>MAAAVTVEEVRRAQRAEGPATVLAIGTATPANCVYQADYPDYYFRITKSEHMVELKEKFKRMCDKSQIRKRYMHLTEEILQENPNMCAYMAPSLDARQDIVVVEVPKLGKAAAQKAIKEWGQPRSRITHLVFCTTSGVDMPGADYQLAKMLGLRPNVSRLMMYQQGCFAGGTVLRVAKDLAENNRGARVLAVCSEITAVTFRGPSESHLDSMVGQALFGDGAAAVIVGSDPDEAVERPLFQMVSASQTILPDSEGAIDGHLREVGLTFHLLKDVPGLISKNIERALGDA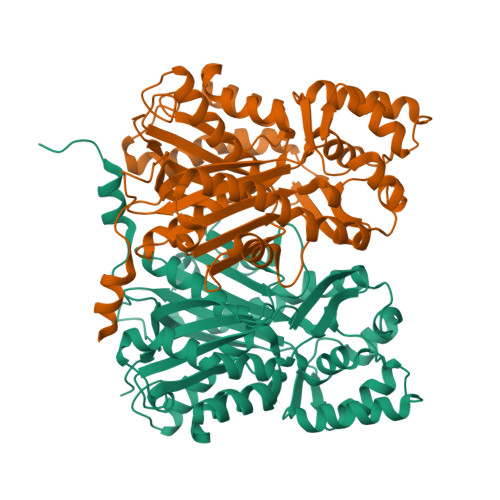FTPLGISDWNSIFWVAHPGGPAILDQVEAKVGLDKERMRATRHVLSEYGNMSSACVLFILDEMRKRSAEDGHATTGEGMDWGVLFGFGPGLTVETVVLHSVPITAGAAA[2x]>HSNEKWFHGKLGAGRDGRHIAERLLTEYCIETGAPDGSFLVRESETFVGDYTLSFWRNGKVQHCRIHSRQDAGTPKFFLTDNLVFDSLYDLITHYQQVPLRCNEFEMRLSEPVPQTNAHESKEWYHASLTRAQAEHMLMRVPRDGAFLVRKRNEPNSYAISFRAEGKIKHCRVQQEGQTVMLGNSEFDSLVDLISYYEKHPLYRKMKLRYPINE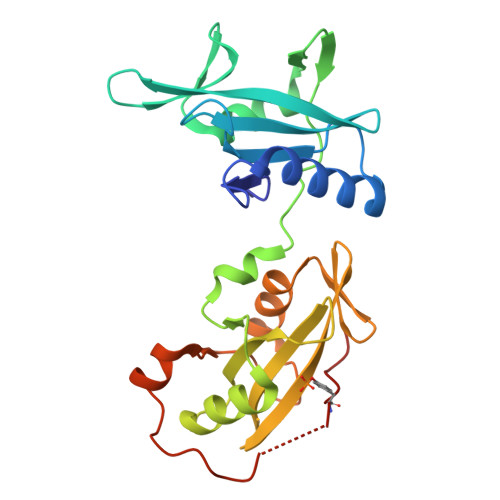EALEKIGTAEPDFGALFEGRNPGFYVEANPMP[4x]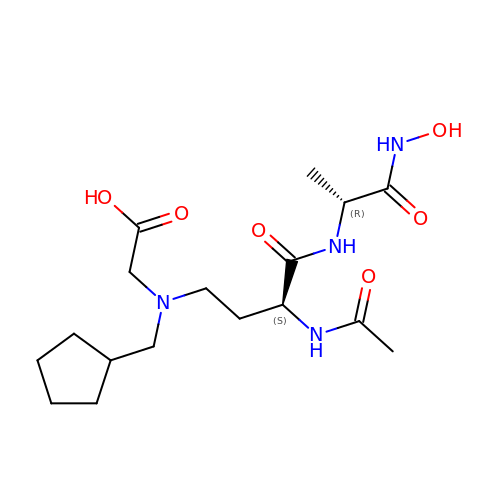2-[[(3S)-3-acetamido-4-[[(2R)-1-(oxidanylamino)-1-oxidanylidene-propan-2-yl]amino]-4-oxidanylidene-butyl]-(cyclopentylmethyl)amino]ethanoic acid | C17 H30 N4 O6 | CZUXSTKXXAXBTE-RISCZKNCSA-N RAR-Related Orphan Receptor C (RORγ, gene name RORC) is an orphan nuclear receptor (NR) that is widely expressed and is involved in regulation of various metabolic processes. RORγ is also a key player in the immune system where the lymphocyte specific isoform RORγt is a so-called ‘master regulator’ of the IL-17 producing T helper (Th17) cell subset. Structural and functional analysis has revealed that the RORγ ligand binding domain (RORγLBD) is comprised of 12 α-helices (H1-H12) and a β-sheet region (BSR) that responds to cholesterol biosynthetic pathway intermediates, hydroxysterols and sterol sulfates. The results presented here indicate that the RORγLBD requires a ligand to stabilize the active conformer and that hyperactivating ligands enhance coactivator affinities by allosterically driving electrostatic intramolecular interactions between H12 and H4.

More recently, RORγ has also been found to be the driver of the androgen receptor in metastatic castration resistant prostate cancer where the selective RORγ antagonist SR2211 elicits a potent cytostatic effect. HDX-MS analysis of the selective RORγ inverse agonist SR2211 revealed a distinctive profile. Specifically, RORγLBD bound to SR2211 exhibited protection to amides surrounding the orthosteric binding site, but SR2211 offered no protection to H12 suggesting that the activation function surface remains disordered. The co-crystal structure solution of the RORγLBD bound to SR2211 reveals a deactivation where the carbinol moiety pushes W317 into an alternative conformation that prevent H11’ and H12 from nucleating. These findings are consistent with previously observed pharmacology and show that HDX-MS measurements can distinguish agonists from inverse agonists.

>ASLTEIEHLVQSVCKSYRETCQLRLEDLLRQRSNIFSREEVTGYQRKSMWEMWERCAHHLTEAIQYVVEFAKRLSGFMELCQNDQIVLLKAGAMEVVLVRMCRAYNADNRTVFFEGKYGGMELFRALGCSELISSIFDFSHSLSALHFSEDEIALYTALVLINAHRPGLQEKRKVEQLQYNLELAFHHHLCKTHRQSILAKLPPKGKLRSLCSQHVERLQIFQHLHPIVVQAAFPPLYKELFSGN[2x]> AMAISITCPPPMSVEHADIWVKSYSLYSRERYICNSGF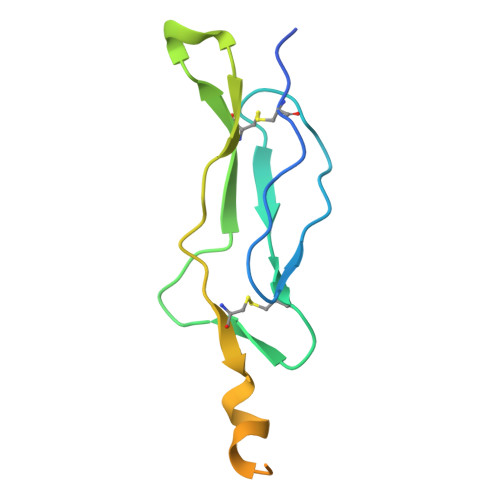KRKAGTSSLTECVLNKATNVAHWTTPSLKCIRDPALVHQRPAPPSTVTTAGVTPQPESLSPSGKEPAAS> MHHHHHHSENTFIFPATFMWGTSTSSYQIEGGTDEGGRTPSIWDTFCQIPGKVIGGDCGDVACDHFHHFKEDVQLMKQLGFLHYRFSVAWPRIMPAAGIINEEGLLFYEHLLDEIELAGLIPMLTLYHWDLPQWIEDEGGWTQRETIQHFKTYASVIMDRFGERINWWNTINEPYCASILGYGTGEHAPGHENWREAFTAAHHILMCHGIASNLHKEKGLTGKIGITLNMEHVDAASERPEDVAAAIRRDGFINRWFAEPLFNGKYPEDMVEWYGTYLNG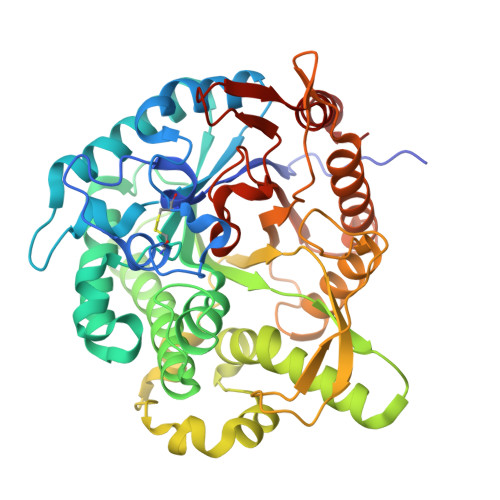LDFVQPGDMELIQQPGDFLGINYYTRSIIRSTNDASLLQVEQVHMEEPVTDMGWEIHPESFYKLLTRIEKDFSKGLPILITENGAAMRDELVNGQIEDTGRQRYIEEHLKACHRFIEEGGQLKGYFVWSFLDNFEWAWGYSKRFGIVHINYETQERTPKQSALWFKQMMAKNGF> MRLTQGCFSFLPDLTDAQIEKQVAYAMAKGWAMNVEWTDDPHPRNNYWELWGLPLFDIKDPATVMFELNEARKSCAA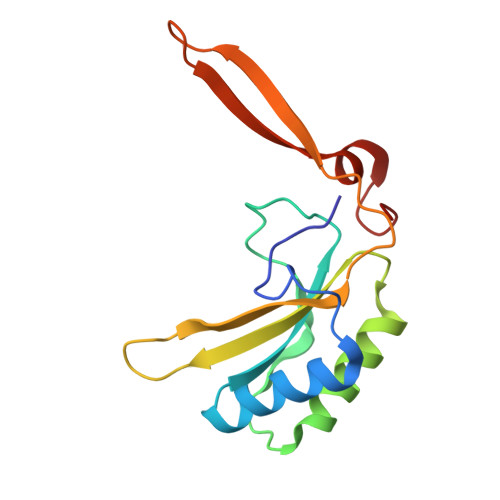GYIRINAFDASYGVESCVMSFITNRPTNEPGFYLDRTDGPGRQIVYSIKSYSVQANPEGSRY> MAKLTALTLLGMGLALFDRQKSSFQTRFNVHREVTPVELPNCNLVKGIDNGSEDLEIL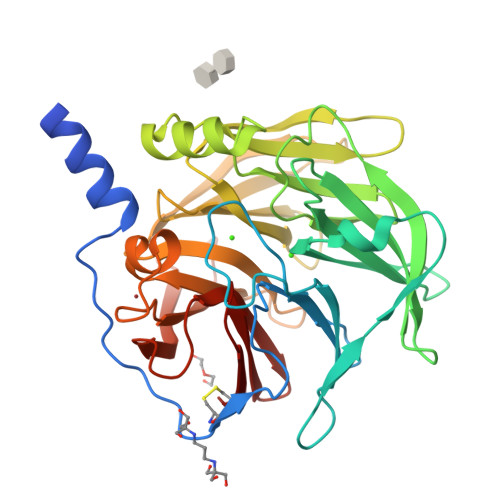PNGLAFISSGGKYPGIMSFDPDKSGKILLMDLNEKEPAVSELEIIGNTLDISSFNPWGISTFIDDDNTVYLLVVNRPGSSSTVEVFKFQEEEKSLLHLKTIRHKLLPSVNDIVAVGPEHFYATNDHYFIDPYLKSWEMHLGLAWSFVTYYSPNDVRVVAEGFDSANGINISPDGKYVYIAELLAHKIHVYEKHANWTLTPLRVLSFDTLVDNISVDPVTGDLWVGCHPNGMRIFFYDAENPPGSEVLRIQDILSEEPKVTVVYAENGTVLQGSSVAAVYKGKLLIGTVFHKALYCDL> GPHMIRYNRDTLMTARDTKRAPIP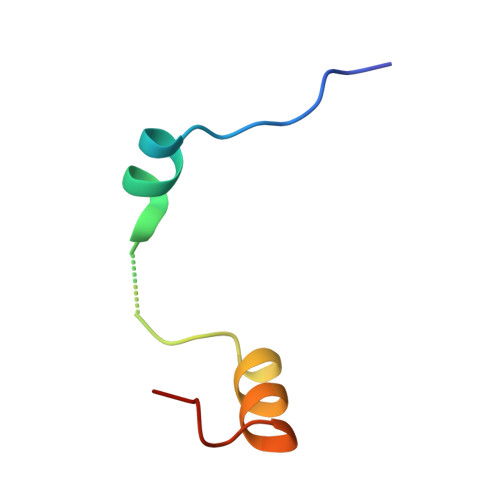DEMLQEINRVAPDILIA[(2~{R},3~{S},4~{R},5~{R})-5-[2-azanyl-5-[[[4-[6-(ethylamino)-5-(2-piperidin-1-ylethylcarbamoyl)pyridin-2-yl]-2-fluoranyl-phenyl]carbamoylamino]methyl]pyridin-1-ium-1-yl]-3,4-bis(oxidanyl)oxolan-2-yl]methyl dihydrogen 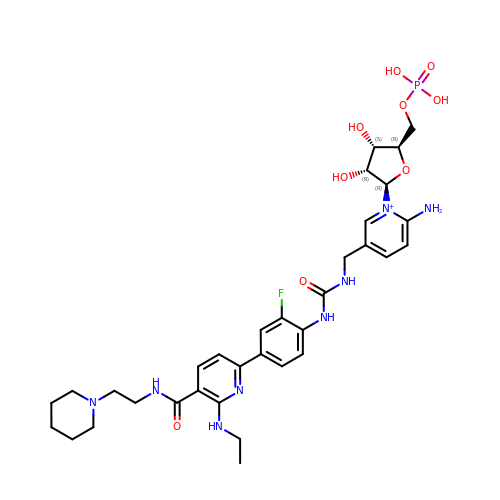phosphate | C33 H45 F N8 O9 P | AJNBKKWBUIHYFX-DWCTZGTLSA-O> GPLGSAAAVESVVSDETLSSNPLLQDFDFPPFDSVDASHVRPGIRALLQHLEAELEELEKSVEPTWPKLVEPLEKIVDRLTVVWGMINHLKAVKDTPELRAAIEDVQPEKVKFQLRLGQSKPIYNAFKAIRESPDWSSLSEARQRLVEAQIKEAVLIGIALDDEKREEFNKIEQELEKLSHKFSENVLDATKKFEKLITDKKEIEGLPPSALGLFAQAAVSKGHENATAENGPWIITLDAPSYL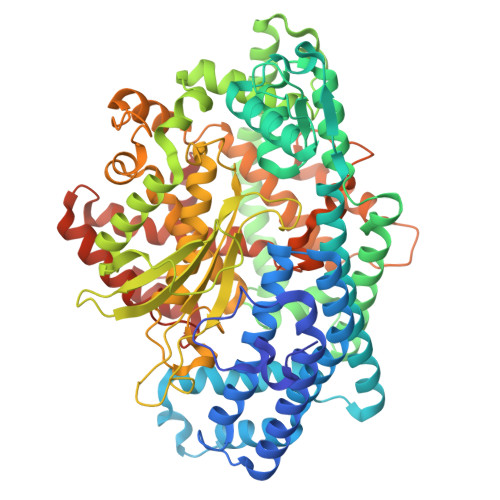PVMQHAKNRALREEVYRAYLSRASSGDLDNTAIIDQILKLRLEKAKLLGYNNYAEVSMAMKMATVEKAAELLEKLRSASWDAAVQDMEDLKSFAKNQGAAESDSMTHWDTTFWSERLRESKYDINEEELRPYFSLPKVMDGLFSLAKTLFGIDIEPADGLAPVWNNDVRFYRVKDSSGNPIAYFYFDPYSRPSEKRGGAWMDEVVSRSRVMAQKGSSVRLPVAHMVCNQTPPVGDKPSLMTFREVETVFHQFGHALQHMLTKQDEGLVAGIRNIEWDAVELPSQFMENWCYHRDTLMSIAKHYETGETLPEEVYKKLLAARTFRAGSFSLRQLKFASVDLELHTKYVPGGPESIYDVDQRVSVKTQVIPPLPEDRFLCSFSHIFAGGYAAGYYSYKWAEVLSADAFSAFEDAGLDDIKAVKETGQRFRNTILALGGGKAPLKVFVEFRGREPSPEPLLRHNGLLAASASA5-(1H-benzimidazol-1-yl)-3-{(1R)-1-[2-(trifluoromethyl)phenyl]ethoxy}thiophene-2-carboxamide | 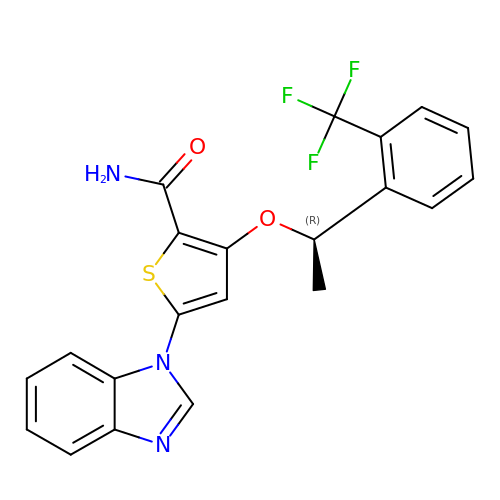C21 H16 F3 N3 O2 S | SQYKBXHMNBHADB-GFCCVEGCSA-N>[2x]XMNASDFRRRGKEMVDYMADYLEGIEGRQV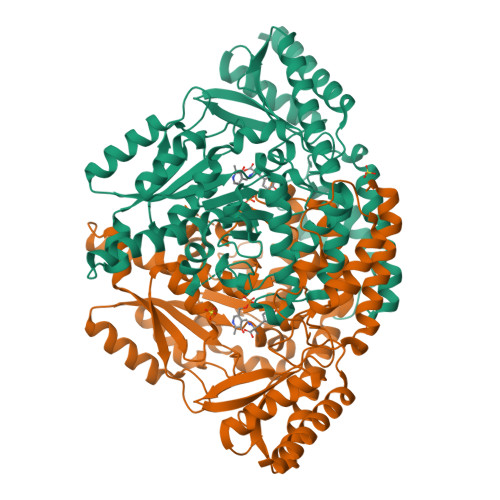YPDVQPGYLRPLIPATAPQEPDTFEDILQDVEKIIMPGVTHWHSPYFFAYFPTASSYPAMLADMLCGAIGCIGFSWAASPACTELETVMMDWLGKMLQLPEAFLAGEAGEGGGVIQGSASEATLVALLAARTKVVRRLQAASPGLTQGAVLEKLVAYASDQAHSSVERAGLIGGVKLKAIPSDGKFAMRASALQEALERDKAAGLIPFFVVATLGTTSCCSFDNLLEVGPICHEEDIWLHVDAAYAGSAFICPEFRHLLNGVEFADSFNFNPHKWLLVNFDCSAMWVKRRTDLTGAFKLDPVYLKHSHQGSGLITDYRHWQLPLGRRFRSLKMWFVFRMYGVKGLQAYIRKHVQLSHEFEAFVLQDPRFEVCAEVTLGLVCFRLKGSDGLNEALLERINSARKIHLVPCRLRGQFVLRFAICSRKVESGHVRLAWEHIRGLAAELLAAEEGKAEIKS> MQFEERLQQLVESDWSLDQSSPNVLVIVLGDTARKYVELGGLKEHVTTNTVAGHVASRERVSVVFLGRVKYLYMYLTRMQAQANGPQYSNVLVYGLWDLTATQDGPQQLRLL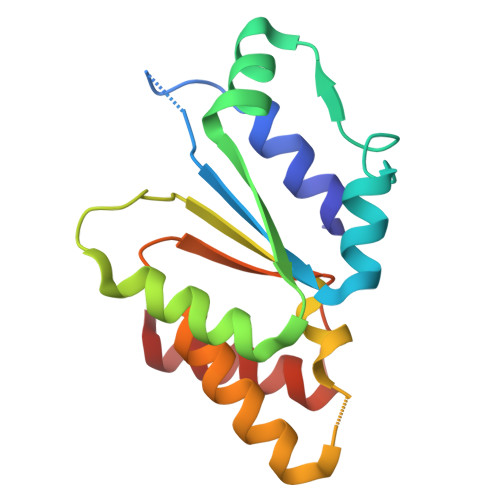SLVLRQCLSLPSKVEFYPEPPSSSVPARLLRFWDHIIR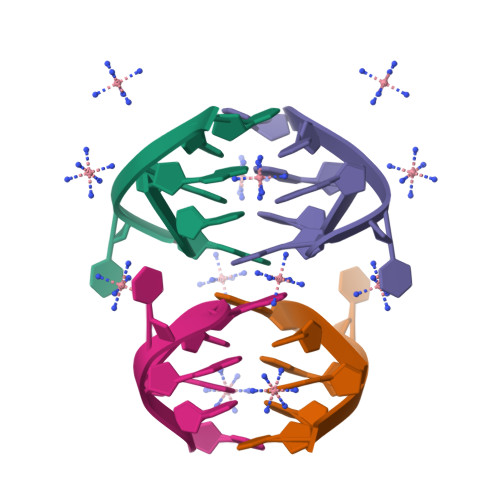>[2x]GCATGCT>[2x]MGSSHHHHHHSSGENLYFQGSHMKAIKL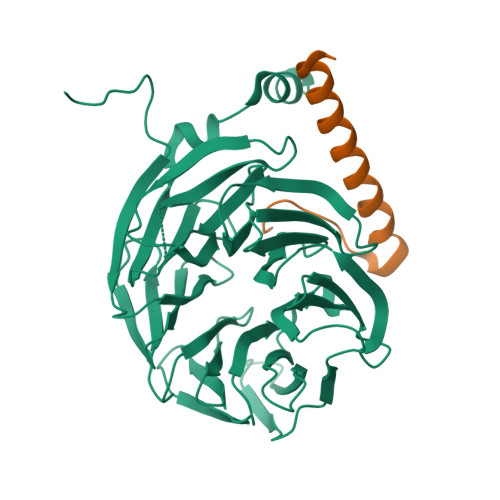TGHERPLTQVKYNKEGDLLFSCSKDSSASVWYSLNGERLGTLDGHTGTIWSIDVDCFTKYCVTGSADYSIKLWDVSNGQCVATWKSPVPVKRVEFSPCGNYFLAILDNVMKNPGSINIYEIERDSATHELTKVSEEPIHKIITHEGLDAATVAGWSTKGKYIIAGHKDGKISKYDVSNNYEYVDSIDLHEKSISDMQFSPDLTYFITSSRDTNSFLVDVSTLQVLKKYETDCPLNTAVITPLKEFIILGGGQEAKDVTTTSANEGKFEARFYHKIFEEEIGRVQGHFGPLNTVAISPQGTSYASGGEDGFIRLHHFEKSYFDFKYDVEKAAEAKEHMQEAN;>GSHMEADTAMRDLILHQRELLKQWTEYREKIGQEMEKSMNFKIFDVQPED[2x]>[6x]LFKPNYHFFPITGWMNDPNGLIFWKGKYHMFYQYNPRKPEWGNICWGHAVSDDLVHWRHLPVALYPDDETHGVFSGSAVEK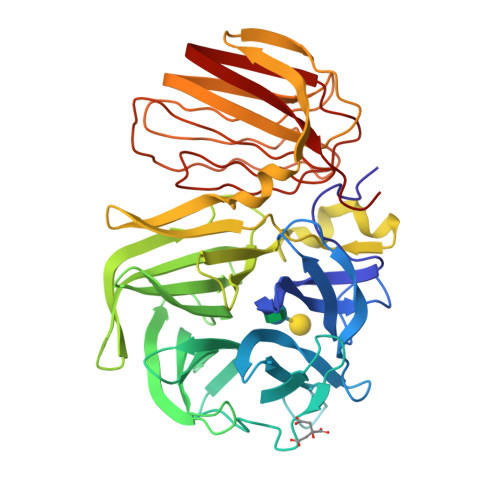DGKMFLVYTYYRDPTHNKGEKETQCVVMSENGLDFVKYDGNPVISKPPEEGTHAFRDPKVNRSNGEWRMVLGSGKDEKIGRVLLYTSDDLFHWKYEGAIFEDETTKEIDCPDLVRIGEKDILIYSITSTNSVLFSMGELKEGKLNVEKRGLLDHGTDFYAAQTFFGTDRVVVIGWLQSWLRTGLYPTKREGWNGVMSLPRELYVENNELKVKPVDELLALRKRKVFETAKSGTFLLDVKENSYEIVCEFSGEIELRMGNESEEVVITKSRDELIVDTTRSGVSGGEVRKSTVEDEATNRIRAFLDSCSVEFFFNDSIAFSFRIHPENVYNILSVKSNQVKLEVFELENIWL> MTVRKNQATLTADEKRRFVAAVLELKRSGRYDEFVRTHNEFIMSDTDSGERTGHRSPSFLPWFRRFLLDFEQALQSVDSSVTLPYWDWSADRTVRASLWAPDFLGGTGRSTDGRVMDGPFAASTGNWPINVRVDSRTYLRRSLGGSVAELPTRAEVESVLAISAYDLPPYNSASEGFRNHLEGWRGVNLHNRVHVWVGGQMATGVSPNDPVFWLHHAYVDKLWAE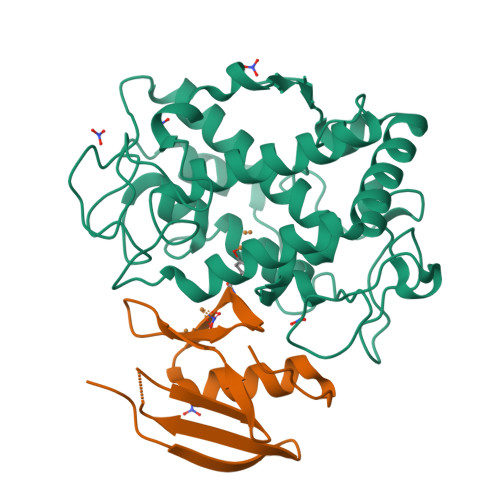WQRRHPDSAYVPTGGTPDVVDLNETMKPWNTVRPADLLDHTAYYTFDALEHHHHHH;> MPEITRRRALTAAAAVAATASAAVTLAAPAASAAGHHEPAAPESFDEVYKGRRIQGRPAGGGAHHHEHGGGYEVFVDGVQLHVMRNADGSWISVVSHYDPVPTPRAAARAAVDELQGAPLLPFPANLEHHHHHH>[2x]MPLGRQSHRHHRTHG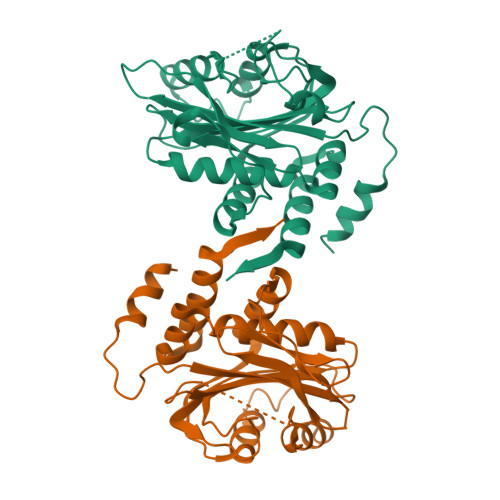QKHRRRGRGKGASQGEEGLEALAHDTPSQRVQFILGTEEDEEHVPHELFTELDEICMKEGEDAEWKETARWLKFEEDVEDGGERWSKPYVATLSLHSLFELRSCLINGTVLLDMHANSIEEISDLILDQQELSSDLNDSMRVKVREALLKKHHHQNEKKRNNLIPIVRSFAEVGKKQSDPHLMDKHGQTVSPQSVPTTNLEVKNGVNCEHSPVDLSKVDLHFMKKIPTGAEASNVLVGEVDILDRPIVAFVRLSPAVLLSGLTEVPIPTRFLFILLGPVGKGQQYHEIGRSMATIMTDEIFHDVAYKAKERDDLLAGIDEFLDQVTVLP3-[4-[5-[4-[[4-(acetamidomethyl)piperidin-1-ium-1-yl]methyl]-6-[3,5-bis(chloranyl)phenyl]pyridin-2-yl]oxypyridin-2-yl]piperazin-1-ium-1-yl]propanoate | C32 H39 Cl2 N6 O4 | 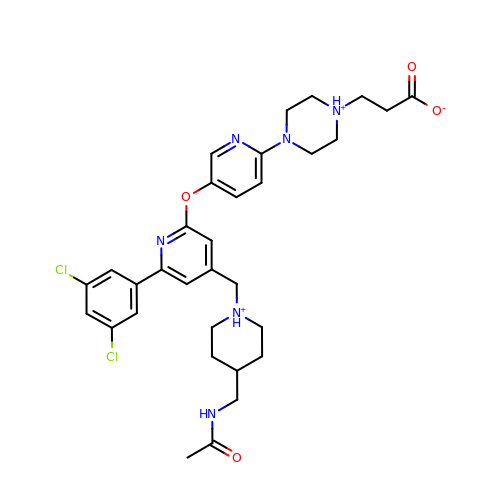YLKNCNAEPRSZSL-UHFFFAOYSA-O>STTGIIMENVTAFWEEGFGELLEKVQQSNGDRKHSSDENNVSFSHLCLVGNPVLKNINLNIEKGEMLAITGSTGSGKTSLLMLILGELEASEGIIKHSGRVSFCSQFSWIMPGTIKENIIFGVSYDEYRYK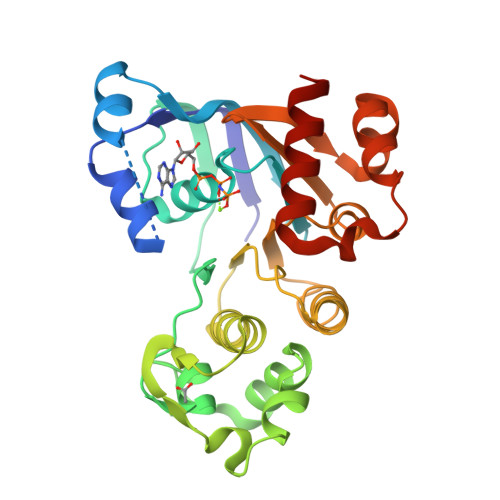SVVKACQLQQDITKFAEQDNTVLGEGGVTLSGGQRARISLARAVYKDADLYLLDSPFGYLDVFTEEQVFESCVCKLMANKTRILVTSKMEHLRKADKILILHQGSSYFYGTFSELQSLRPDFSSKLMGYDTFDQFTEERRSSILTETLRRFSVDD[4x]> GSTLVTGSEYE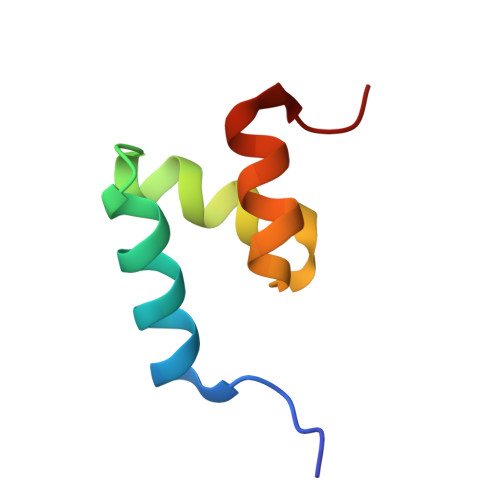TMLTEIMSMGYTRERVVAALRASGNNPHRAVEYLLTGIPG>MSRRPTLRLGLDRDVYNIVLNLEQQGTDENGKRPRLTVDYVYDTIKRSNSSLARQKKRMLEDSIERVLAVRKEQAKAEEETDSDDLIEAQERERERQKAAQAQRDANLLNRQIAKSWGFASSPGAKAADGEKGTDTGSIATPAPATPAVAENMAADTPTTSTGPVLPASSTDRQPNGEPRPKKRKAAPKEIDRTPPTKVSILDIAGVDDTLQRLLKEVWFPLRGGEACEKMGYRYDNGVLLHGPSGCGKTTLAHAIAGSIGVAFIPVSAPSVIGGTSGESEKNIRDVFDEAIRLAPCLIFLDQIDAIAGRRESANKGMESRIVAEIMNGMDRIRQNTPLGKNVVVLAATNRPEFLDPAIRRRFSVEIDMGMPSERAREQILRSLTRDLSLADDINFKELAKMTPGYVGSDLQYVVKAAVSESFQANIDSLLAQARAKHPADHLANVSQPQRDWLLLEAHRDEEVSWPSTKITMEQFRKAVSLVQPASKREGFSTIPDTTWSHVGALEDVRKKLEMSIIGPIKNPELFTRVGIKPAAGILLWGPPGCGKTLVAKAVANESKANFISIKGPELLNKYVGESERAVRQLFSRAKSSAPCILFFDQMDALVPRRDDSLSDASARVVNTLLTELDGVGDRSGIYVIGATNRPDMIDEAIRRPGRLGTSIYVGLPSAEDRVKILKTLYRNTVKAPKKREGTNGEDVDMTDAAAEQQHQGTTDADLEKVALDLRCTGFSGADLGNLMQAAAQACLERVYTQRQQKRKEGGSVAEEEEIEPVITMEDWEKALNEVKPSVKDPEKYMHSGFAAALEHHHHHH[6x]

Rix7 is a poorly characterized type II AAA-ATPase that plays an essential role in the assembly of the large ribosomal subunit. Rix7 is a type II AAA-ATPase, composed of a unique NTD followed by tandem well conserved AAA modules known as the D1 and D2 domains respectively. Rix7, the earliest acting ATPase, is proposed to drive release of the essential ribosome assembly factor Nsa1 from nucleolar pre-60S particles. In summary, our work establishes Rix7 as a nucleolar molecular unfoldase that utilizes the D1 and D2 AAA domains to thread substrates through its central pore via a processive hand-over-hand mechanism.

To determine the full-length structure, we utilized single particle cryo-EM to obtain an electron scattering map of a Chaetomium thermophilum Rix7 double Walker B mutant (CT Rix7E303Q/E602Q) and derived a structural model of the hexamer. The EM data were classified and refined without imposing symmetry which resulted in one dominant conformation at 4.5 Å resolution, that contained well resolved density for all 12 AAA domains. The electron scattering map revealed that Rix7 adopts an asymmetrical stacked hexameric ring configuration composed of six subunits of Rix7 (referred to as protomers P1-P6). The cryo-EM reconstruction lacks density for the entire NTD of Rix7 (amino acids 1-192), suggesting that this domain is flexible and dynamic. There is sufficient density within the pore to accommodate a ~20 residue unfolded peptide spanning the entire 80 Å length of the pore across the D1 and D2 domains. Five of the six protomers (P1–P5) within both the D1 and D2 domains grip the polypeptide through their pore loops, while P6 does not contact the peptide. The Rix7 cryo-EM structure reveals that even in the absence of the aromatic-hydrophobic-glycine motif, PL-I within the D1 domain of Rix7 (h-S-G, where h is a hydrophobic residue) grips the polypeptide. We defined the P6 protomer as the seam subunit because it does not contact the polypeptide or closely pack with the neighboring AAA domain thereby creating a seam or break in the hexameric ring. In the D1 AAA domain, ATP is present in the nucleotide pockets of all six protomers, whereas only four nucleotides were observed in the nucleotide binding pockets of P1-P4 from the D2 AAA domain. There is no density for ATP in the nucleotide binding pocket of P5 from the D2 domain.> GKPKRPRSAYNVYVAERFQEAKGDSPQEKLKTVKENWKNLSDSEKELYIQHAKEDETRY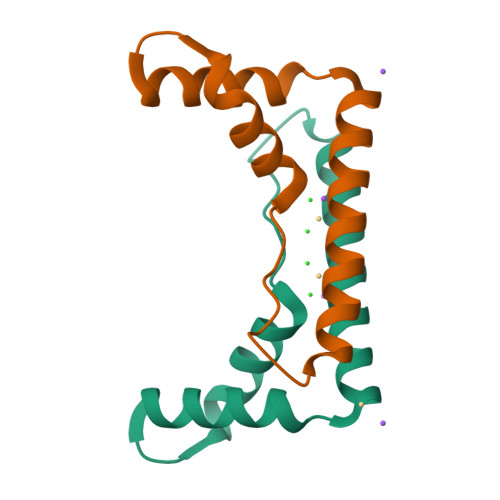HNEMKSWA> LVHVASVEKGRSYEDFQKVYNAIALKLREDDEYENYIGYGPELVRLAWHISGTWDKHDNTGGSYGGTYRFKKEFNDPSNAGLQNGFKFLEPIHKEFPWISSGDLFSLGGVTAVQEMQGPKIPWRCGRVDTPEDTTPDNGRLPDAD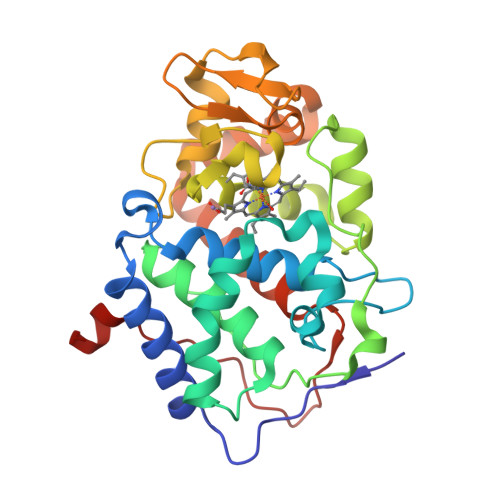KDAGYVRTFFQRLNMNDREVVALMGAHALGKTELKNSGYEGPWGAANNVFTNEFYLNLLNEDWKLEKNDANNEQWDSKSGYMMLPTDYSLIQDPKYLSIVKEYANDQDKFFKDFSKAFEKLLENGITFPKDAPSPFIFKTLEEQGL Purple acid phosphatases belong to the family of binuclear metallohydrolases and are involved in a multitude of biological functions, ranging from bacterial killing and bone metabolism in animals to phosphate uptake in plants. Plant PAPs are 110 kDa homodimers, containing Fe(III)-Zn(II) or Fe(III)-Mn(II) centers, and a recombinant isoform from sweet potato has been shown to contain a di-iron center. The characteristic purple color is due to a charge transfer transition between a tyrosine side-chain and the Fe(III). In this study the structures of the rkbPAP-sulfate and rkbPAP-fluoride complexes were determined, providing insight into what we propose are two crucial steps in its catalytic mechanism, (i) the pre-catalytic stage, and (ii) the chemical step.

In this study rkbPAP was co-crystallized with sulfate, and diffraction data were collected at a resolution (2.4 Å) which is better than that for any previously determined plant PAP structure. The Fe(III) and Zn(II) in this structure are separated by an average distance of 3.1 Å, similar to that reported for the other rkbPAP structures. Spherical electron density is observed 2.1 Å from Fe(III) and 2.3 Å from Zn(II) and therefore in a bridging position. We therefore assign this density to that of a μ-hydroxo group, an interpretation in agreement with a previous study involving measurements of the magnetization of rkbPAP under catalytically relevant conditions. The Fe(III) is coordinated by a nitrogen atom from the side chain of His325, oxygen atoms from the side chains of the chromophoric Tyr167, Asp135, Asp164 (which bridges both metal ions), and the bridging hydroxide. Zn(II) is also pentacoordinate, ligated by the side-chain oxygen atoms of Asp164 and Asn201, the side-chain nitrogen atoms of His286 and His323 and the μ-hydroxide. Mechanistically, it is important to stress that the μ-hydroxide group is the only water molecule present in the active site, and given the location of this group the fitting of a sixth ligand to either metal is implausible. In contrast to the phosphate-bound rkbPAP structure, the sulfate ion in the active site does not coordinate directly to the metal ions. Instead it is positioned in the second coordination sphere, stabilized via an extensive hydrogen bond network involving His202, His295, His296 and the Zn(II) ligand Asn201. Thus, the rkbPAP-sulfate complex demonstrates, for the first time, how the pre-catalytic complex predicted from stopped-flow measurements may be formed and stabilized in the second coordination sphere of the enzyme.

>RDMPLDSDVFRVPPGYNAPQQVHITQGDLVGRAMIISWVTMDEPGSSAVRYWSEKNGRKRIAKGKMSTYRFFNYSSGFIHHTTIRKLKYNTKYYYEVGLRNTTRRFSFITPPQTGLDVPYTFGLIGDLGQSFDSNTTLSHYELSPKKGQTVLFVGDLSYADRYPNHDNVRWDTWGRFTERSVAYQPWIWTAGNHEIEFAPEINETEPFKPFSYRYHVPYEASQSTSPFWYSIKRASAHIIVLSSYSAYGRGTPQYTWLKKELRKVKRSETPWLIVLMHSPLYNSYNHHFMEGEAMRTKFEAWFVKYKVDVVFAGHVHAYERSERVSNIAYKITNGLCTPVKDQSAPVYITIGDAGNYGVIDSNMIQPQPEYSAFREASFGHGMFDIKNRTHAHFSWNRNQDGVAVEADSVWFFNRHWYPVDDST[2x]>[2x]MASHHHHHHSGMEEWNFPVEYDENYLPPADSRYWFPRRETMPAAERDKAILGRLQQVCQYAWEHAPFYRRKWEEAGFQPSQLKSLEDFEARVPVVKKTDLRESQAAHPPFGDYVCVPNSEIFHVHGTSGTTGRPTAFGIGRADWRAIA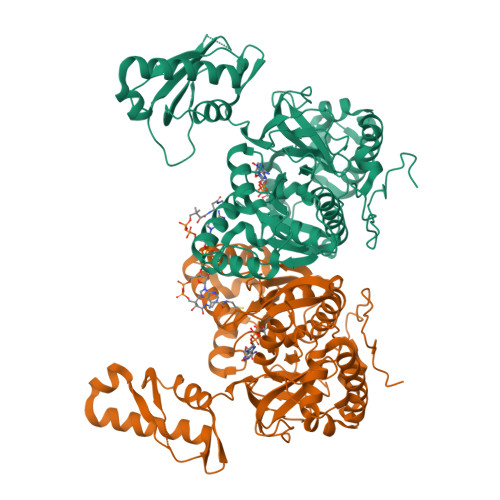NAHARIMWGMGIRPGDLVCVAAVFSLYMGSWGALAGAERLRAKAFPFGAGAPGMSARLVQWLDTMKPAAFYGTPSYAIHLAEVAREEKLNPRNFGLKCLFFSGEPGASVPGVKDRIEEAYGAKVYDCGSMAEMSPFMNVAGTEQSNDGMLCWQDIIYTEVCDPANMRRVPYGQRGTPVYTHLERTSQPMIRLLSGDLTLWTNDENPCGRTYPRLPQGIFGRIDDMFTIRGENIYPSEIDAALNQMSGYGGEHRIVITRESAMDELLLRVEPSESVHAAGAAALETFRTEASHRVQTVLGVRAKVELVAPNSIARTDFKARRVIDDREVFRALNQQLQSSAGSAWSHPQFEK>[2x]DPATCEK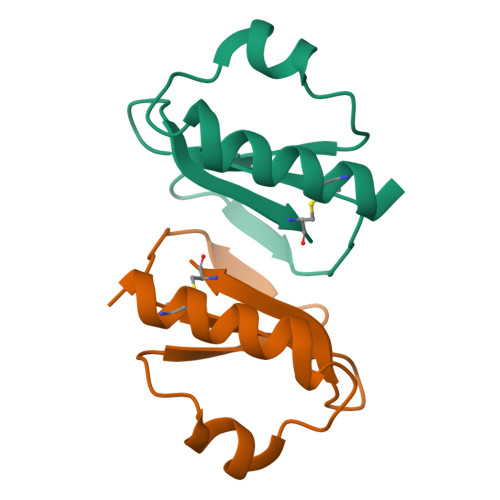EAQFVKQELIGQPYTDAVANALQSNPIRVLHPGDMITMEYIASRLNIQVNENNEIISAHCA 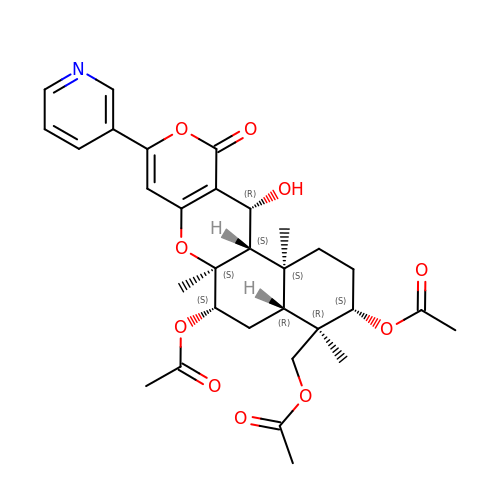(3S,4R,4aR,6S,6aS,12R,12aS,12bS)-4-[(acetyloxy)methyl]-12-hydroxy-4,6a,12b-trimethyl-11-oxo-9-(pyridin-3-yl)-1,3,4,4a,5,6,6a,12,12a,12b-decahydro-2H,11H-naphtho[2,1-b]pyrano[3,4-e]pyran-3,6-diyl diacetate | C31 H37 N O10 | PMMQOFWSZRQWEV-RVTXXDJVSA-N>[2x]SIGTRWAVLIAGSKGYHNYRHQADVCHMYQILRKGGVK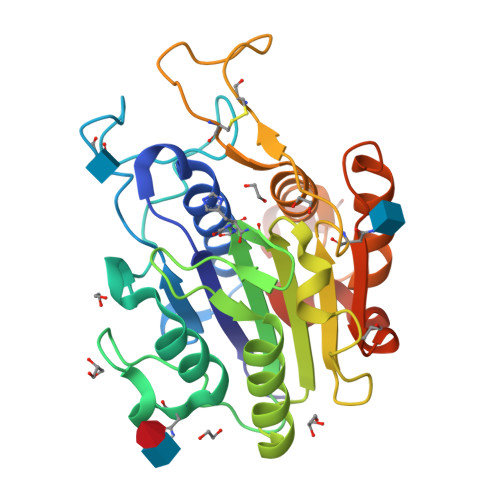DENIIVFMYDDIAYNESNPFPGIIINKPGGENVYKGVPKDYTGEDINNVNFLAAILGNKSAIIGGSGKVLDTSPNDHIFIYYAXGAPGKIGMPSKPYLYADDLVDTLKQKAATGTYKSMVFYVEACNAGSMFEGLLPEGTNIYAMAASNSTEGSWVTYCPGTPDFPPEFDVCLGDLWSITFLEDCDAHNLRTETVHQQFELVKKKIAYASTVSQYGDIPISKDSLSVYMGTDPANDNRTFVDEN> GPLGSWVIPPISCPENEKGPFPKNLVQIKSNKDKEGKVFYSITGQGADTPPVGVFIIERETGWLKVTEPLDRERIATYTLFSHAVSSNGNAVEDPMEIL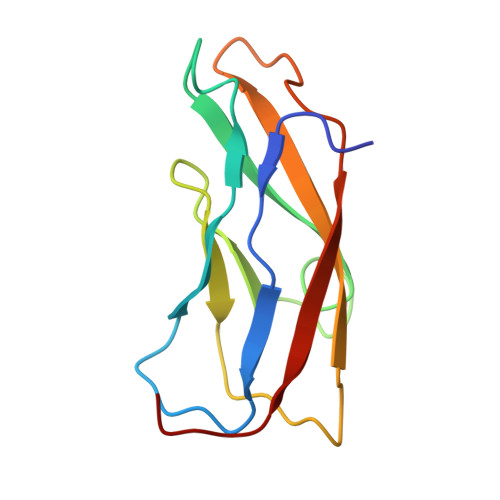ITVTDQNDN> MMVIDTSALVAMLSDEPDAERFEAAVEADH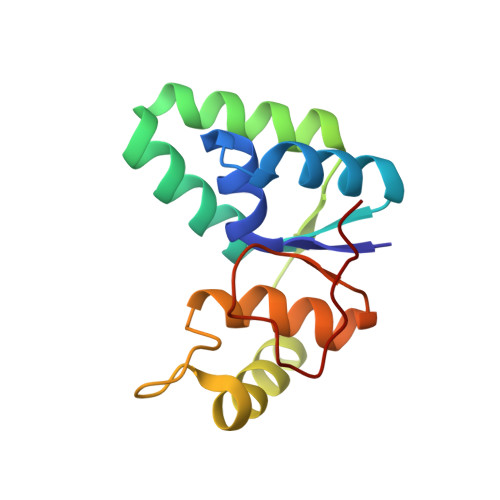IRLMSTASYLETALVIEARFGEPGGRELDLWLHRAAVDLVAVHADQADAARAAYRTYGKGRHRAGLNYGDCFSYGLAKISGQPLLFKGEDFQHTDIATVALP> GSHAPIHARMQQLVSEFQNTLDALDSVIASRLMQMALEAARQVIGQTPAVDNSALIKQIQQLL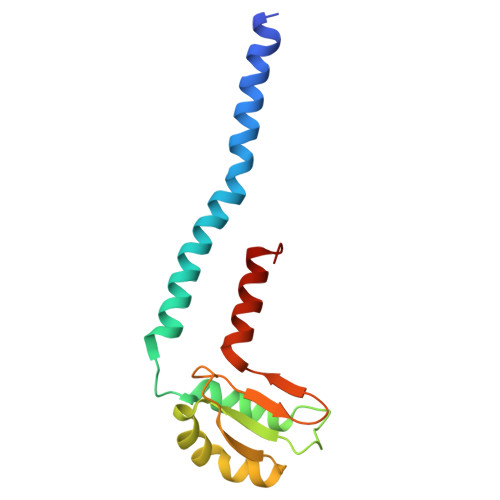QQEPLFSGKPQLRVHPDDLQRVEEMLGATLSLHGWRLRGDPTLHHGGCKVSADEGDLDASVATRWQELCRLAAPGVL> MNITIYDVAREANVSMATVSRVVNGNPNVKPTTRKKVLEAIERLGYRPNAVARGLASKKTTTVGVIIPDISSIFYSELARGIEDIATMYKYNIILSNSDQNMEKELHLLNT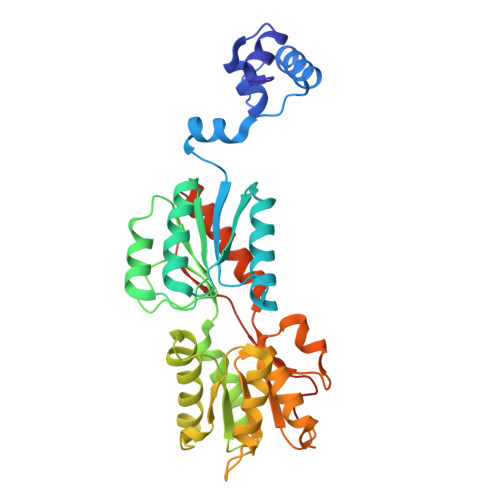MLGKQVDGIVFMGGNITDEHVAEFKRSPVPIVLAASVEEQEETPSVAIDYEQAIYDAVKLLVDKGHTDIAFVSGPMAEPINRSKKLQGYKRALEEANLPFNEQFVAEGDYTYDSGLEALQHLMSLDKKPTAILSATDEMALGIIHAAQDQGLSIPEDLDIIGFDNTRLSLMVRPQLSTVVQPTYDIGAVAMRLLTKLMNKEPVEEHIVELPHRIELRKSTKAHHHHHH>AQTYEITYQNSFEGKINPNQNHIISITNSDKTLLFNEKIKNKKADFPFEVNEINRKNNEVSQFAFLNNNEIVKTSDNTILAKQEFKPTSETGKILGYNVKKAVTSVNSNTIEVWYTNDLKVKGGPSILGQDLGLVLKTVRNGSSVVEATSVKKIKALDDQSLFNGKNITEKDALTYKDMIWKSRFITIPVFENETINFSDASKSDQVIQRFGNGTIILKKVKIPEIKQGNTIFVELKQKSNGDAYDRTGDVFIIPQERAISYYTGLTQGVKSLPVYQNGNGKSYQGVALTPDYLPFIELMRFFTPFGIGHFNEKIQLKGKNWHNNTPYRQDITELRPQLSGKEILIGAFIGNYDKGGHQISLELSIHPDQQKIVNNNFVLPVFNTTNVMEMAGQDYPTMFNSDKGVEVEFILTKDLKNAQLRYITTGHGGWGAGDEFVPKENSIYLDGKLAHAFTPWRTDCGSYRLFNPASGNFEDGLSSSDLSRSNWCPGTITNPVYINLGNLNAGKHTIQV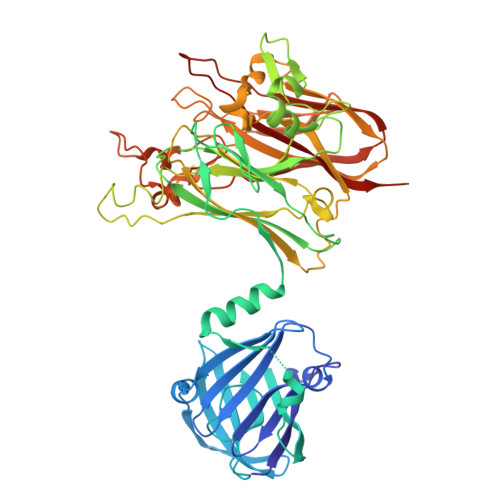KIPQGAPEGSSQSFWNVSGVLLGQEHHHHHH[4x]>MGRENVLPVHNDVYEDFVFTTPYFQPESTFKSVPKLFSDILLGGVEWVYTTSESVLAYDYKLWYLWSGVSNLDESFDMFFNQYWALSLSTSVFQLFYAVILDRYLSVLFQNTPYTNDWFRMMLHSKETALIWLYHPELSWHINGLNQFFTYFYGGILEFVYFDKSNPDMCILVHTLWIHLLILFLIFTGFVTILFSFYGNPNTEENTIDSDYLAASGTVEAEKEITSIDDYLGLVFAIAYVFGVFFYVHGWTSMLSHAVLLLSCYSIIIMFLFILGMPTLLLYDFGIFFLAYLKGAGKYISSVAEMMFDYTACLVFYIRILAQWIRVVLMVVTFISLSHYVSDFDITNSALIGSENQSDSMNELNTNFSMTYYILTVLPGKFIYWIYEILHTFFVVCSQFVAFFAIVFWLFLFLYTFFIIEKHEDFFSKKREERKKKLKELWNLKN[2x];>[2x]MHSTLRVFTKNNCLSFTNMNRFSTAAQVAQANYSKFRADYSASVAAFQQRIKTIEKENTGSMKKPMAKAYEHPYNSEHHPLNFSAVKIAETFHDFIGPEQVSPHYESFAMSRKFLLTFWGGFFVLNFGMATVDLNWIMKSTYIPWIFWFQLMYFYVEGKNSMFMPLLQRFYRRAAANEIFTMEAFYHENIENKLRNLMRITKGQLEYWDIHTSYGEIRADSINNFLANEYLRLQSHITSRALNILKQAQAYETMNQAALLQKLIDDATSAIDNALKGDKKAEVLARSLDSAIDGLSKGYMDYQNDPLLPLILSSIEANVKKITTLSAQEQANLIGLTAEQLKSIKENDVRARKEFLESQPKLDNNLKNIESVKKILATWGK;>[2x]MITILDYLFLLDLNDDLTRKAVFEQVIIFIFIYCTMNFLAWSTVVELIWPTHFFNRRHSSSQEFIRFRTYTEVLLKISAYNDFFYVLNNYYYNQKLILKN;>MSMLAKIAKNVVKTQALKNTTAAQTPSFQAPGNQDKILKWISTLSNKATTGESRSYCTQLSSLVSFYNKQHVEQIPTIDFNEWKSVISTQGLVDKVKENYESLIKEQYNTDAISKQISSASSKALDDIENELSFHAAIWLNAYADYTMFLFELEEYNDPNDYLMHENFDFFRGLETELEELTETHNYIPGAKDDVNLRGYLATQFAWGKKVISFYRHPADDFKCAKATKNMLGR[2x];>[2x]MIHCLRNIRTVSALQSKISYNLGGGNKRKKTSGDLDNYDVLFVGANLGGICSNHFDKDTHGKYKCFVSFDQPINQIYSVRIPYEQQRVRKSEYIHFSKKSINQFTPSEMLAVKEILPEQNAVVLSSGRRIGYNQLVLATGLKHDFSQIKGFYEALEHPEHPVYANRDPETWRSAQHKYSKYISNFKSGDGYFCIPEYPYAGEVECFNFFVSDEVWKWAQHHGALSPKHTFTIVNANEKFVHYCDSADAFIKERLEKRGIRVEYNTKLLEVHQDGQKATFINTKTGEKSVRDYNNLYSIVPSKRQEFLDKAGLTNGNGLLNVDHQTLQHKKYKNIFGLGDAADLPTTKTFWAGWYQIAVVRNNVKRNLQGQTLNAHYDGFSKVPLFTGHQTLTYVAHSYGGVGNWQHLKHNNGGILAWMRYRSWAKGMAKKFQDFYNGARLGPPYHKVLKSFPELPGSPESQQSSGISKYFPTKTENKAAH;>[2x]MSLHEKMQTDYLWVKDHSQADSWAKARTHGYNYIAHTVPNKKERYEMIWRSMGKSTDWELEKFRLGKKFPDRGNKRRWFKNLFRLIKNPMGYIFWKTYKARLAKPSLIVTSMFIGFTLGFIKLKAQSIAYSKKQYATLRAGKNIEGSGQVHFGYHDQKWGMPAIPMFQLMYYELPGNSIVVNPCRNQNYRLYFEMRKKLGILPA;>[2x]MINRSTAFISKNLRQANLTQSSLAMKTQYNQMGFSSDNPYNKRWEYKWKHSYYTYPRDYEHTEVRKPQDSKDVPPIYFAYYKDFVDRWLPGMNMWWQRRHRIFDKFNVYFLPGMSLFFYQFADLALGFKIMAAFPLFLAYTRIRDKTLDPDFKETYLRDMIYQNPEITKYFNEETIHVLDYEFEYLPGYLCPEKFPEYQNKTWQFFNTDTAQAEGFFKFGDVESGATMTLKFKTMPIPGKFRYQVGEPFYFYDLRAEIKCDGVYKEVVLVDEKESLKKIRPFLFLI;>MQQRKKIYLRQKRKIYIQLKNKEKKKNNQFIQKREKMGYKIRNKSIFWTRAGWKNNWHPKNFNAPRPSYGEFTMGIRCRNDHHSFLRYVQTYRNMSRHCKQYFLGDKQLEETFILGLRSLFLVPYDSQCLTDQIKHGGERRFVDQLDRDFELISYNTHPYQLFTYTVRNEHLAWKNEQYEKIQKGEKTFEQELLDYLDEQVLAEKAKLRDGQNFSIERMTEIALHVFRKARAGKVRPAQDVRGPDGNVNDFLEQRRPFEHPNPTGVTH[2x];>[2x]MNPIQKAWLKILEPVSYVINEKMAKRTGIIGKLGRFFAIGPREYGVHPINRMFIFMNRKYMAFQAVALHRYSFVKSLTHNGFHMLRVFRHFAFVLPATVLAGLGLFVYWGDDNKCYSPDRFPYLKKRAGDMALPLNSLNQRTSAHYIEINAIYGAEMMKRYHKVWENIIEERSKATDQEKKTRYAHPSYQYSPLPVVSIPNVLNPLNLQ;>[2x]MSENKAPGQIYAYDIHNTHYPYVNIKQDSQTQLLASFRRSIASINPFSYRQVPSQDRAAFGLRWGNAWYAPNPYPNGIHFDRVFPTHYDPLAETNRTKANLQLIKYAPGNYSTLVVTSEKLPRPCIRTIQNYRRCQMVNGTEKCNSEAQDILAICPNWALDHMKEKVRFYTKALAINNQTYIRAMQVEEYNQGRTVADVAPKTWIHGTRQHLRPDTMWADDRYTNITQTEINEAIKRVEARKAREHEKKPVEQANVNANTGEQPVRVEKSLYP;>[2x]MWYKYFSKQSWNLRVWRKANLKYNQDDFGMTQPKYIARFGDFRFRLVRTEGALRGCMFFVGFGCFSIINYLYGRYGYIINESSQKRAAQDLLDNDMAADKILFKNRVGAPTRPLRSLDDMMAFLSGSATYDQLADYASYNHAMDVNQDQQAGLDSWMSEKDKNMVKYYQRSLGKKVEGI;>MPVKEGQAKLWFSTKEEADAYDDKMISNIELKSQDYEDENFSPVFNRKTQEYFLEPSEKFKSDFAELLRPLRSLSFNQVVDRYVLIPPNHTFYRNWTYEKFLGGFGLSYLILRELPLRNFYARVFVMYAFAAKVLDHLGNPFPFSGHGQIVAAADRWNHWDVRCYDNVMKALKYIRIPTVQNNIPEATRWYGRQPGHLLRADTYWIPNLVSQRFAKHQPAHWDGTQNMPIFRLADPKHKDSYMVQFR[2x];>MDNYFTAITLLGLRDQNLPPFKDARLQRYKSIKKMIDLIETTTKLAPPMPVELFMLNPTDPEWDDDMTYPTITHATALYKSSALAGNLFLYAYNYNNFTANIRLRTMRYLFPVVSLAIFGNIYWDYRSQLVKVNLFDEYIQARAQELVKQNEYLLEHEDVKRYVWWYEDLKETLARVHRQANNHKACDFKDSEIILQDFIRRYTNPKDNLPIKFHPQGQTF[2x];>[2x]MEGFIQNKRKKEKEGEEEEESKEKRKQINQLNKQKQEEEKIYQQKKDQKRKKYLYQRKEMTIFAETWEASEYQYRNKANLKTLPVNHLGKLAELKFDFVEYKAHQLIACHLYERMTIHCMNQYGLFKDFYRPECLDAQYYFKTCVELNAAYGIQKKFFPEHFVGSPYARPVPQFQQLGL;>[2x]MKQKINKLLKNKGVQDKYKYLSKLILLDQEIKGKIKRKNKKEKQKRKNKLILEEMQNTTNIVHVPVHMGHTHYFDYIDSFPKLKEGPTLEENHITNQKILREQLISGQQGLEQNLCLRNCFKLSQKRYIEFCLDRKCGGADFQRAATILGYTKN;>MSNIFLELQDGDKTVYTHTSLIEESKQEQIQAIYDKVPQWTNGGRFLGFWLSMEAVNRVQSVAKLPIYYRAGIVATSTLLGGLVSSLVFWKSGNENQVAKLANGAPVYLKKWEVPELSKLYFFLDDDNNFKPSLNHHAVTQGRQYYKIYQHN[2x];>[2x]MFRNILSLVTKPSKLSQKTFYNFAAAKNEVQVSKKQQQAGAKRDLTQYVEGQIVNRNQLTLKKQEDIEQYVLKLVRGYFRTTNKQGLNINSVLQDHGLDEFDSIELAMQVEEDLGYVISAETIPVLNKVKHFVNYINHV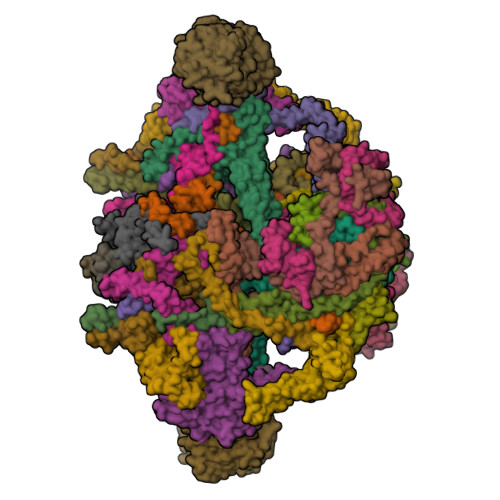EQFKAENGKAPIA;>MSQDPKIVNPQLWPNPNKLRFADLYKYQGVEMKKINDSIKNYKAAKFYIGGILGGCLVFKFFIDAAVDKYIFGENGNGGKFLEMQTINSNYDYYYNRQFQRMRYLTEDPAGDDPLQKTKDEHLVDLGFIPKVFGANVEVRKRAPHDKYL[2x];>[2x]MNSLSSKKANSLVFKSIRNFTLQWGSLAERPMVDRVMSTSTWPVPYYQRLFKAYPIREKKDKMSLLLSDIDIDDTNWYQAKDFLRGSFRGRQIVDYVENNIASNTYILIQQDVANMAKAYVHDICGYIDVANKENVRILSKGDLI;>[2x]MNRSVNIAKNLIQTYRAMSVQSRFAFSTREEEWLDKRTKSQEKVYFDQEDRKAMKRLLEKLNTTSKFVEDSEYLAPQNLEVENILKRYHINYTQALIDELVDWKTGKN;> MKMEYLQSEEKKDAINKQIHKKEEKEEKEIKIKRKNKVKQRIQIINQIKKYIEAKQQKKQIQSKNQRKYKGRMINTRKQVFKCLWGAQPAYNFSRIINHLRGDPVYQDNTKDVSLRGTFLRGKYDDLPTMIFFTEACDLTANWIPFFTNPQYDILAHRNVWLLNPRNFGNSDRHPSFDLQEMSDDVMRFMYSQKISMATLGGHGIGGKIALAVGCYHAERVTGVFSIDSSPMDQRYHEAFKEFKGYVNALTEINFKTWSDKDVKVFLKENIKDPKWRSIFTNNISKNAKTQSDSFNFEINYLNHNLNFNKADSLGNWAVKNGIYTGRAHFIFPEYSRWVHLATNTLPMHKVCARVKGFGHDIFYVQGDENPLNHWVYDFENYANVVASKLNKFLHSYDGVHALLKDRTEIGNFMIPDRIKSRNDSKHIYGDYSPAHLHHNWRFNHIYEKHDELDKKLNEQ> MTEQFLKDNFSLEGKVALITGASYGIGFSIATAFARAGATIVFNDIKQELVDKGISAYKKLG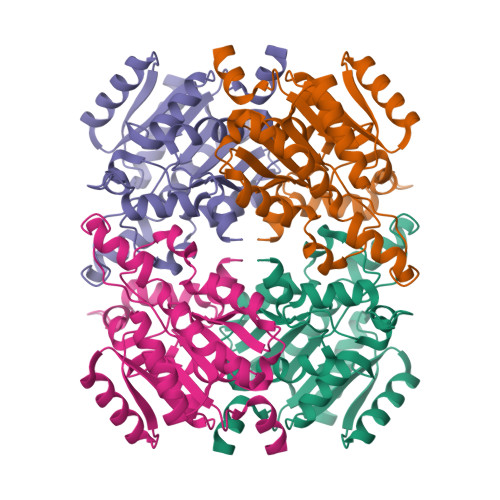IKAHGYVCDVTDEDGINEMVDKISQDVGVIDILVNNAGIIKRTPMLEMSAADFRQVIDIDLNAPFIVSKAVLPGMIQKGHGKIINICAMMSELGRETVAAYAAAKGGLKMLTKNIASEYGSANIQCNGIGPGYIATPQTAPLRERQDDGSRHPFDQFIIAKTPAARWGEAEDLGAPAIFLASDASNFINGHILYVDGGILAYIGKQPQLEHHHHHH4-{4-[(4-methoxyphenyl)methyl]phenyl}-1,3-thiazol-2-amine | C17 H16 N2 O S | 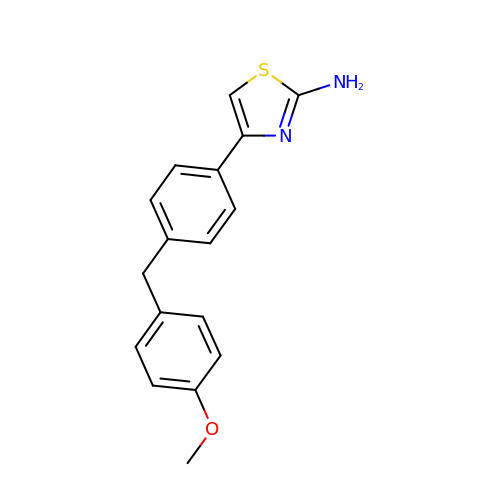GGCCOFFVKJCRKJ-UHFFFAOYSA-N>[2x]MAKDK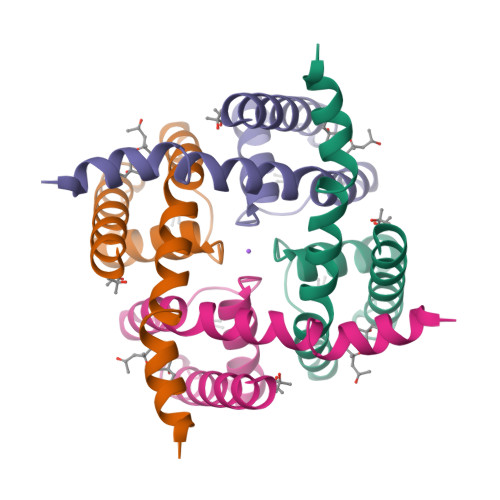EFQVLFVLTILTLISGTIFYSTVEGLRPIDALYFSVVTLTTVGDTPPPQTDFGKIFTILYIFIGIGLVFGFIHKLAVNVQLPSILSNLVPR> MGSSHHHHHHSQDPMEIDELTALGGLLHDIGKPVQRAGLYSGDHSTQGARFLRDLAENTGRAEYELLSLFSEFHHKGHMKNDELMIRRIKELSPERFGLTMEDVLNALWIVYEADNLASGEREEGQPQASRPLYSVFNPGKAYPWAELDFEKELPVPGD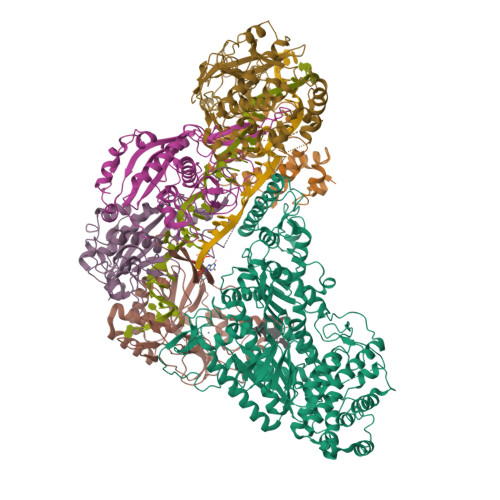VFSIRSQDYRELVKRLWEELSKAKLRSDRLLPVLEKYLTFVSSVTSEGNIISLYDHMRMTSAIALAMLRAGCTAEDVRSGRCRKEKRFLLIEGDFSGIQDFIYRVSGKGTLKYLRARSAYLELIGWDVVLEILSRLGLTRANVVFNAGGHFMIIAQNTPDAVKELEEIRAKAVEWLYREFESDLYLAIEWEPVSGREFGREGGKNLFAEARKRLKHKLTVRKLKRFGEIKGLFEHGHTERLAECPVCGRELPEGKLEPSASDPETKVCPTCNRLVSLGGNLPKLLGFGRTAKNDAGVLVEGPFSGFVPYLQGGRPVGEQILVKNTLNPGEIPESAQFVPYFVADYFKKDPKGGVATFEELSMASTGTRRLGVMKGDVDRLGEFFSSMDSPSKLATASRFMDYFFKGYIGAIIEGKFGYIIGDVPSLRDWPEEPDIVVVYAGGDDFFIVGAWDQIFELAFRVRRAFNAYTGGKLTLSVGLGYFDERTPIYRMADVVSERLDTAKDEGRNRVFVVGRSRPLDGKHKLSYEWNHYEELWRTYAPRIYAGNGRLKGKLESKKGLLWKLLEIRELYVRDPNDVRWAYLTAYLLGRHGLSDLFPELVGIDTKAVERKEPQPVYWVDGVLKIVLMAVRR;> GSVAYHQKHGGYGRGGYGRQDRPQVDASRLFGESPDVVGIKKMLEGKGKQWEAIQPYFDNVVREAKNFLEWSPNKRLANAVTVAAYLTSQGLKTNQVRKILDMARTTELKVKRGEGDIKDDLVKMRYLLAYTVGKATGQSKYSLDAFHRILDPMLEVLMGSPKKENFEKFYDFLQAVVAYHKFFGGGD;>[2x]GSMDRRFYGKIVIKGKIKAVTGLHIGSQRDISEIGGIANPVIKDPHTGLPYIPGSSLKGRLRSLFEILVNSRLGEWREKYPSLANYSPGSCRPDNQENCGKFFNRKINRGWIHVCPDYETALACPVCRLFGASGKESNFPSRIIVRDAFLTKEWEEKWRAGEAITEAKIEVGIDRVTSQANPRTNERVVAGAEFEFEIIYNVENTTHWRDDIKNLLTAMALLEDSYLGGSGSRGYGKVKFIFDSFEFRPLDYYRTGKDEDIVSIDAREKSVSDILSGFDSLFSEVEGKLEAG;> MPKFIAVKLIPKGPFRDIPRADTLFGAIGNAISAIHGQSAVEELVDAFVGGARISSAFPYSGDTYYLPKPLSVEPALEGILTGLDEEERYTTAKRLRKAKYLDLKNFELALRLRPFTIPEEIPYARVDVPRVVLDRVTQDSSIYFWEEIRFREKSGVYFLYSGPREVFDGYIAPAMRFLGDTGIGGKSTWGAGLFEVEFHEMKIDAPGSEYSVTLSNALPTKTPVLWRLLRKGGWSFGRRKPRMTFIAEGSIVKNDPGGMERLELGLSHEVYVYGLTFPLGVELPEGLE>GILELAGTVGCVGPRTPIAYMKYGCFCGLGGHGQPRDAIDWCCHGHDCCYTRAEEAGCSPKTERYSWQCVNQSVLCGPAENKCQELLCKCDQEIANCLAQTEYNLKYLFYPQFLCEPDSPKC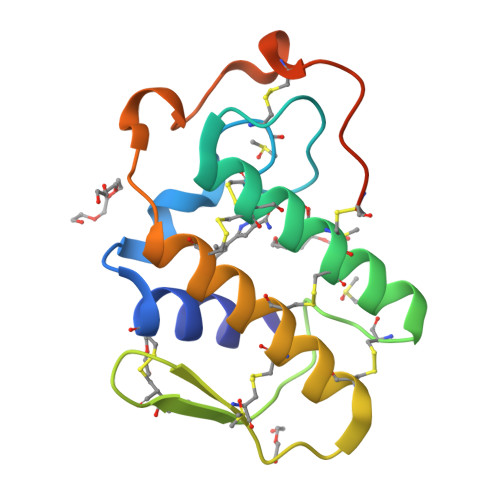DQGILELAG[2x]>[4x]MGSSHHHHHHSSGLVPRGSHMCNSDNTSLKETVSSNSADVVETETYQLTPIDAPSSFLSHSWEQTCGTPILNESDKQAISFDFVAPELKQDEKYCFTFKGITGDHRYITNTTLTVVAPTLEVYIDHAS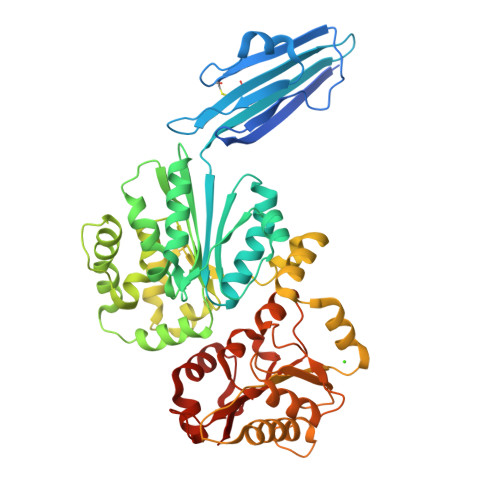LPSLQQLIHIIQAKDEYPSNQRFVSWKRVTVDADNANKLNIHTYPLKGNNTSPEMVAAIDEYAQSKNRLNIEFYTNTAHVFNNLPPIIQPLYNNEKVKISHISLYDDGSSEYVSLYQWKDTPNKIETLEGEVSLLANYLAGTSPDAPKGMGNRYNWHKLYDTDYYFLREDYLDVEANLHDLRDYLGSSAKQMPWDEFAKLSDSQQTLFLDIVGFDKEQLQQQYSQSPLPNFIFTGTTTWAGGETKEYYAQQQVNVINNAINETSPYYLGKDYDLFFKGHPAGGVINDIILGSFPDMINIPAKISFEVLMMTDMLPDTVAGIASSLYFTIPADKVNFIVFTSSDTITDREEALKSPLVQVMLTLGIVKEKDVLFWA>GEFMVSIMLLKVEDLHVYRGNREILKGVNLTVEENEIHAIIGPNGAGKSTLAYTIMGISGYKPTKGRIIFKGVDIIDKNITERARMGMTLAWQEPARFEGIKVKNYLMLGMNEKYKKDKEIAEEKIREALKLVNLDPDKYLDRYVDETLSGGERKRIELASIICMEPDLAILDEPDSGIDIVSFDEIKRVFDYLKDKGCSLLVITHREELAEHADRVSLICAGEVIKSGDPKEVGEFYKKECGKCYKKVPDGK[2x];>[2x]GEFELMSIKEELMEIIEAIKYTSEKPEEIVHGKGPRIIVKESRIIDVQGDEGIILEGKEEDGKIKAKIIVKKGYKFKYPIHMCFGITEENISQIIDVEIILEEDSSISLMSHCSFPKGKGIKHIMNGIIKIGKNAKFSYNEFHYHGMDGDILVKPTVKVEIDEGGIYISNFTLTKGRIGTLDIEQEIIAKKDAIIDITTRTYAIKEDVVKVNEVVKLNGENAKCIIKSRGAAMDNSKISLKLKIEGNAPYSKGHIDCAEIVKGNAEVESIPIVVVRDDKARITHEAAIGSVDKKQLETLMAKGLDEDEATEIIVKGMIGDL

The present study focuses on the ancestor SMS from the hyperthermophilic archaeon Methanocaldococcus jannaschii. Biochemical and structural studies showed that SMS is made of a SmsC2B2 heterotetratmer wherein the SmsC subunit hosts both ATP and [Fe-S] cluster binding sites. With respect to the six components of the SUF system, SMS has only two components, SmsC and SmsB, encoded by the smsCB operon. The SmsC subunit, consisting of a RecA-like domain and a helical domain, contains all the structural motifs of the nucleotide-binding (NBD) subunits of the ABC ATPases (i.e., Walker A, Walker B, ABC signature, D-, Q-, and H-loops).

Since attempts to crystallize a [Fe-S] cluster-bound protein complex either in the absence or in the presence of AMP-PNP were unsuccessful, we used cryo-EM to determine its structure. The reconstituted SmsC2B2 complex prepared for crystallization in anoxic conditions, was rapidly vitrified for cryo-EM single particle analysis, and the structure determined reached a global resolution of 2.64 Å. The protein complex prepared in these experimental conditions revealed that the C-terminal residues C218, C239, and C242 of one SmsC subunit coordinate a [4Fe-4S] cluster. These three cysteine residues bind the cluster in a solvent-exposed hydrophobic pocket consisting of residues P40, L216, I223, Y235, and P247. Although the SmsC2B2 complex could in principle contain two such binding sites at the SmsC head-to-tail dimer interfaces, the two SmsC subunits form a strong asymmetric dimer with a single populated [Fe-S] cluster binding site. All residues coordinating the cluster and forming the hydrophobic pocket are in a single SmsC chain. In contrast with the unoccupied SmsC subunit (apo-SmsC), the [Fe-S] cluster-bound SmsC displays a folded C-terminal α-helix composed of residues 227–241 and a short terminal loop. This region comprises the two-cysteine motif (-C239-G240-K241-C242-) coordinating the [Fe-S] cluster, and P247 closing the hydrophobic pocket. Additionally, residues of the C-terminal region extend the dimeric interface between the apo-SmsC and [Fe-S] bound SmsC subunit, in the vicinity of the cluster binding site. This interface consists of a cation–π interaction between the side chains of the K128 in apo-SmsC and the Y243 in [Fe-S] bound SmsC, as well as the side chain-backbone intermolecular hydrogen bonds from the N131 in apo-SmsC and the K236 in [Fe-S] bound SmsC.The mammalian TRPC subfamily consists of seven transmembrane proteins (TRPC1-7) that have been proposed to form non-selective cation channels in various cell types. TRPC6 and its most close homologs TRPC3 and TRPC7 are unique among the TRPCs in that they can be directly activated by second messenger diacylglycerol (DAG), a product of phospholipase C action. TRPC6-mediated cation influx regulates physiological function of pulmonary endothelial cells, smooth muscle cells and glomerular podocytes, whereas TRPC6 hyperactivity has been implicated in maladaptive tissue and organ remodeling. In this study, we present two high-resolution cryo-EM structures of antagonist- and agonist-bound human TRPC6 in lipidic nanodiscs.

Detergent-solubilized TRPC6 (Δ2–72) was first purified to homogeneity in the presence of the antagonist AM-1473, and then exchanged into lipidic nanodiscs composed of the membrane scaffold protein, MSP2N2, and soybean lipids. The structure of the antagonist-bound TRPC6 in nanodiscs was determined at a resolution of 3.1 Å using single-particle cryo-EM (Table 1 and Figure 1—figure supplements 2–3). Based on the shape and chemical environment, it is very likely that the density within the pocket of S1-S4 observed in the final postprocessed map and two corresponding half-maps belongs to the antagonist AM-1473, which consists of an aminopiperidine, a benzonitrile, and an indane. The antagonist engages in both hydrophilic and hydrophobic interactions with residues from S1-S4, the TRP helix and the membrane-reentrant loop following the TRP helix. The primary amine moiety off the piperidine ring forms hydrogen-bond interactions with Glu509 on S2, and Asp530 on S3. The benzonitrile group is involved in a cation-π interaction with Arg758 on the reentrant loop as well as aromatic-stacking interactions with His446 on S1 and Tyr753 on the TRP helix. The indene double ring makes van der Waal contacts with Tyr612 on S4. Overall, the three ring groups in the antagonist knit the intracellular ends of S1-S4, the TRP helix and the reentrant loop together. Mutation R758A, which disrupts the cation-π interaction, lowered the binding affinity by ~300 fold. We found that the AM-1473-bound TRPC6 and the BTDM-bound TRPC6 assume a nearly identical conformation (Cα-RMSD 0.588), with S1-S4 and the S4-S5 linker in the slightly up conformation, distinct from the slightly down conformation in agonist-bound structure.

>AYMFSDRSTSLSIEEERFLDAAEYGNIPVVRKMLEECHSLNVNCVDYMGQNALQLAVANEHLEITELLLKKENLSRVGDALLLAISKGYVRIVEAILSHPAFAEGKRLATSPSQSELQQDDFYAYDEDGTRFSHDVTPIILAAHCQEYEIVHTLLRKGARIERPHDYFCKCNDCNQKQKHDSFSHSRSRINAYKGLASPAYLSLSSEDPVMTALELSNELAVLANIEKEFKNDYKKLSMQCKDFVVGLLDLCRNTEEVEAILNGDVETLQSGDHGRPNLSRLKLAIKYEVKKFVAHPNCQQQLLSIWYENLSGLRQQTMAVKFLVVLAVAIGLPFLALIYWFAPCSKMGKIMRGPFMKFVAHAASFTIFLGLLVMNAADRFEGTKLLPNETSTDNAKQLFRMKTSCFSWMEMLIISWVIGMIWAECKEIWTQGPKEYLFELWNMLDFGMLAIFAASFIARFMAFWHASKAQSIIDANDTLKDLTKVTLGDNVKYYNLARIKWDPSDPQIISEGLYAIAVVLSFSRIAYILPANESFGPLQISLGRTVKDIFKFMVIFIMVFVAFMIGMFNLYSYYIGAKQNEAFTTVEESFKTLFWAIFGLSEVKSVVINYNHKFIENIGYVLYGVYNVTMVIVLLNMLIAMINSSFQEIEDDADVEWKFARAKLWFSYFEEGRTLPVPFNLVPSPKSLFYLLLKLKKWISELFQGHKKGFQEDAEMNKINEEKKLGILGSHEDLSKLSLDKKQVGHNKQPSIRSSEDFHLNSFNNPPRQYQKIMKRLIKRYVLQAQIDKESDEVNEGELKEIKQDISSLRYELLEEKSQNTEDLAELIRELGEKLSMEPNQEETNR[4x]6-[(~{S})-methoxy(phenyl)methyl]-~{N}2-methyl-~{N}4-[(1~{S},5~{R})-3-oxabicyclo[3.1.0]hexan-6-yl]pyridine-2,4-dicarboxamide | C21 H23 N3 O4 | 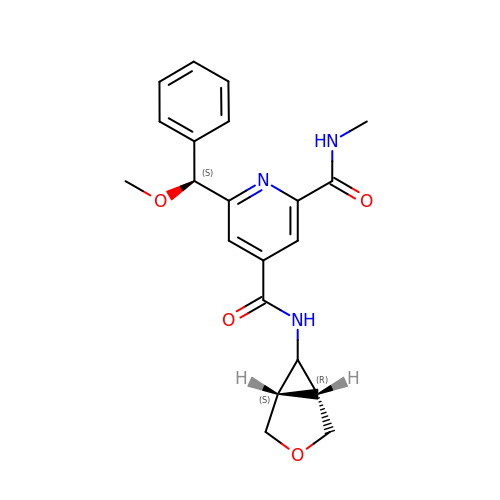XRABYUHHDSKQAA-SFUIVIKGSA-N>[6x]MAKKTSSKGKLPPGPTPLPFIGNYLQLNTEQMYNSLMKISERYGPVFTIHLGPRRVVVLCGHDAVREALVDQAEEFSGRGEQATFDWVFKGYGVVFSNGERAKQLRRFSIATLRDFGVGKRGIEERIQEEAGFLIDALRGTGG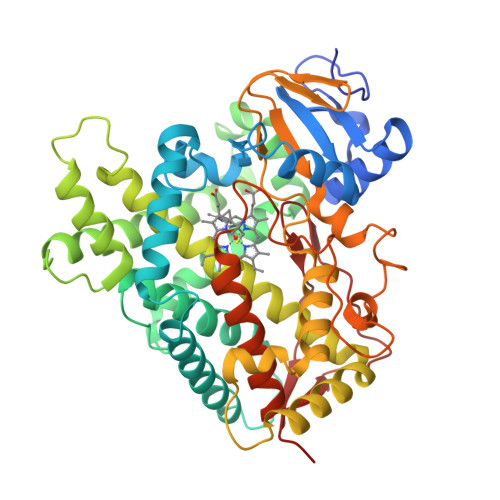ANIDPTFFLSRTVSNVISSIVFGDRFDYKDKEFLSLLRMMLGIFQFTSTSTGQLYEMFSSVMKHLPGPQQQAFQLLQGLEDFIAKKVEHNQRTLDPNSPRDFIDSFLIRMQEEEKNPNTEFYLKNLVMTTLNLFIGGTETVSTTLRYGFLLLMKHPEVEAKVHEEIDRVIGKNRQPKFEDRAKMPYMEAVIHEIQRFGDVIPMSLARRVKKDTKFRDFFLPKGTEVYPMLGSVLRDPSFFSNPQDFNPQHFLNEKGQFKKSDAFVPFSIGKRNCFGEGLARMELFLFFTTVMQNFRLKSSQSPKDIDVSPKHVGFATIPRNYTMSFLPRHHHH ethyl 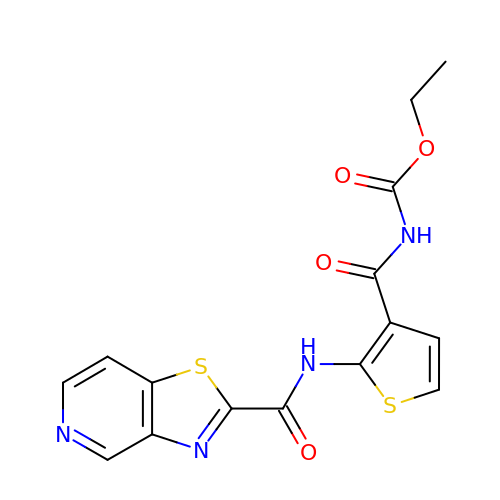{2-[([1,3]thiazolo[4,5-c]pyridine-2-carbonyl)amino]thiophene-3-carbonyl}carbamate | C15 H12 N4 O4 S2 | JCOQDKZVKXILLW-UHFFFAOYSA-N> MSTIFPFIGVPEDYILPKTEELPIFREVAWDFEKDEPILEKGDFKIIEKKEALKVWIYKCIKTNRYEHEIYSLEYGTELSELIGQKYTKGLTESEASRFIKEALLINPYILEVNVKSAN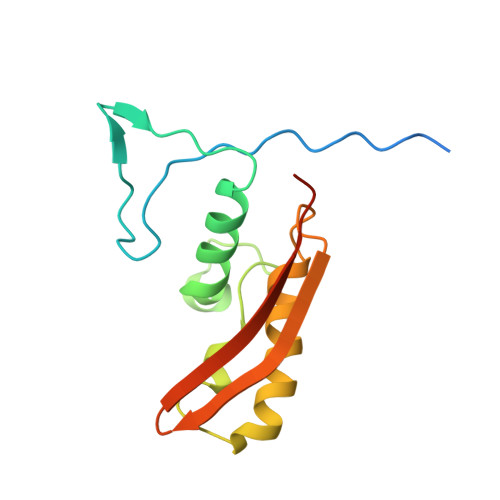FNRDILSANVKVSTIYGEVEINV> GAFLELDVPKADLTIKATGKQWYWSYAYPDNGKFEFDSLMAQDKQPRLLGVD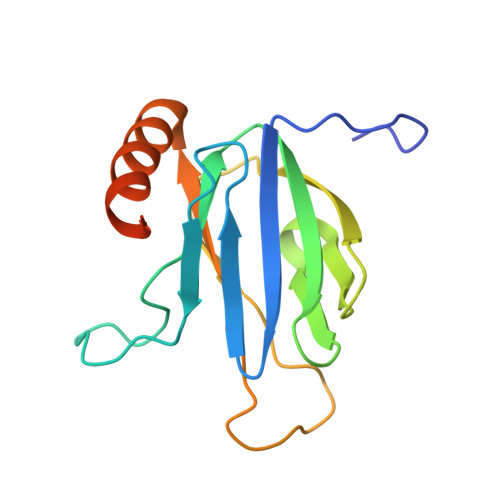NEMVVPVNKVIRVQVTGADVIHAFALPAFGVKIDAIPGRLNETWFKAAKTGMFYGQCSELSGKDHAFMPIAIRVVEDKEFASWVETAKKKFASGGTGTYASAAGPTQ>[2x]GKAFDDGAFTGIREINLSYNKETAIGDFQVVYDLNGSPYVGQNHVSFITGFTPVKISLDFPSEYIMEVSGYTGNVSGYVVVRSLTFKTNKKTYGPYGVTSGTPFNLPIENGLIVGFKGS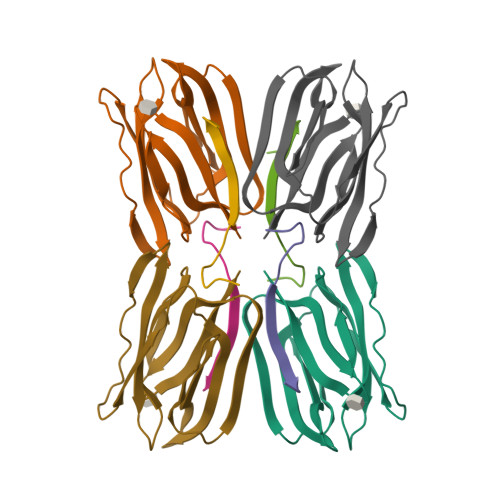IGYWLDYFSMYLSL;>DEQSGISQTVIVGPWGAKSA[4x];>[2x]GKAFDDGAFTGIREINLSYNKETAIGDFQVVYDLNGSPYVGQNHKSFITGFTPVKISLDFPSEYIMEVSGYTGNVSGYVVVRSLTFKTNKKTYGPYGVTSGTPFNLPIENGLIVGFKGSIGYWLDYFSMYLSL> GPSVERTFLPNGNYNIKSIFSGS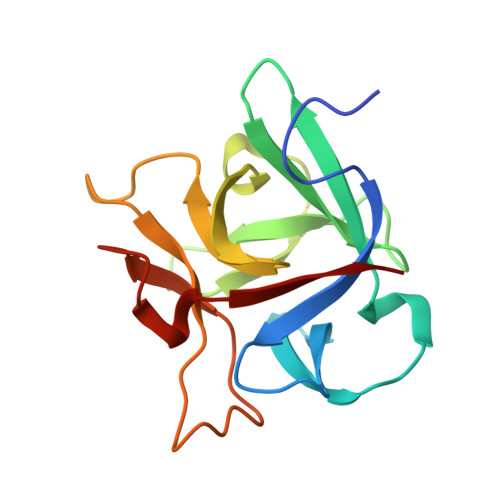LYLNPVSKSLTFSNESSANNQKWNVEYMAENRCFKISNVAEPNKYLSYDNFGFISLDSLSNRCYWFPIKIAVNTYIMLSLNKVNELDYAWDIYDTNENILSQPLLLLPNFDIYNSNQMFKLEKI>EFRPEMLQGKKVIVTGASKGIGREMAYHLAKMGAHVVVTARSKETLQKVV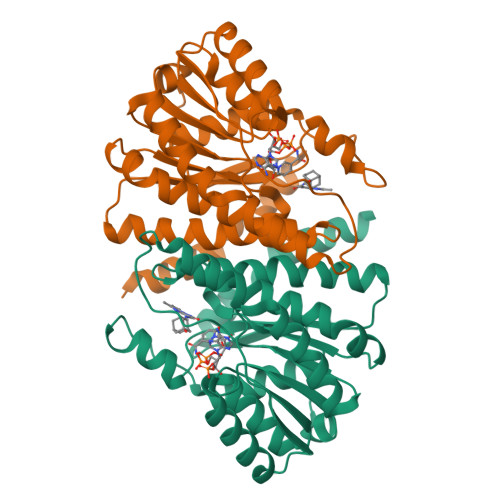SHCLELGAASAHYIAGTMEDMTFAEQFVAQAGKLMGGLDMLILNHITNTSLNLFHDDIHHVRKSMEVNFLSYVVLTVAALPMLKQSNGSIVVVSSLAGKVAYPLVAAYSASKFALDGFFSSIRKEYSVSRVNVSITLCVLGLIDTETAMKAVSGIVHMQAAPKEECALEIIKGGALRQEEVYYDSSRWTTLLIRNPSRKILEELYSTSY[2x]>ARSTDTFNYATYHTLEEIYDFLDLLVAENPHLVSKIQIGNTYEGRPIYVLKFSTGGSKRPAIWIDTGIHSREWVTQASGVWFAKKITQDYGQDAAFTAILDTLDIFLEIVTNPDGFAFTHSTNRMWRKTRSHTAGSLCIGVDPNRNWDAGFGLSGASSNPCSETYHGKFANSEVEVKSIVDFVKDHGNIKAFISIHSYSQLLMYPYGYKTEPVPDQDELDQLSKAAVTALASLYGTKFNYGSIIKAIYQASGSTIDWTYSQGIKYSFTFELRDTGRYGFLLPASQIIPTAKETWLALLTIME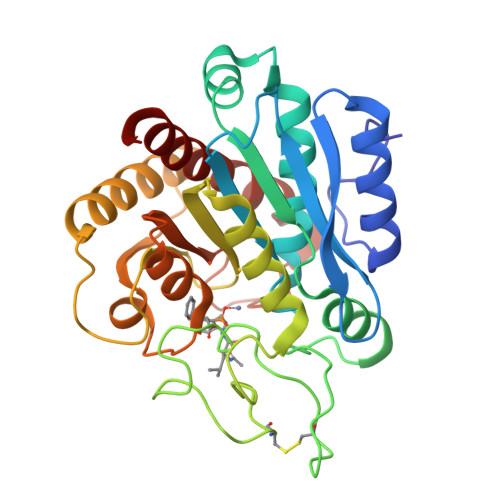HTLNHPY[2x]>MHHHHHHMLENKLGIINQLELNRVEERVSKENAKRLYDSGDIDRIEVGTFKGLSYIHNYLFEDIYEFAGKVRSQNISKGNFRFAPVMYLEIALEHIDKMPQRNLDEIVAKYVEMNIAHPFREGNGRATRIWLDLILKKELKR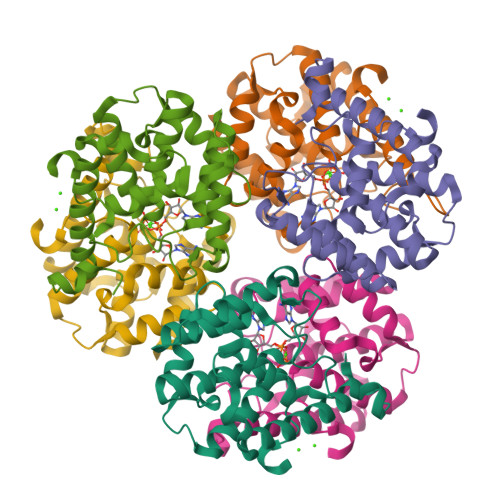VVDWNLINKEDYLSAMERSPVKDLEIKYLISNALTDKINDREIFMKGIDISYYYEGYTEYNVDEL[12x]>MAGSGKFFVGGNWKCNGTKDSIAKLISDLNSATLEADVDVVVSPPFVYIDQVKSSLTDRIDISGQNSWVGKGGAFTGEISVEQLKDLGCKWVILGHSERRHVIGEKDEFIGKKAAYALSEGLGVIACIGEKLEEREAGKTFDVCFAQLKAFADAVPSWDNIVVAYEPVWAIGTGKVASPQQAQEVHVAVRGWLKKNVSEEVASKTRIIYGGSVNGGNSAELAKEEDIDGFLVGGASLKGPEFATIVNSVTSKKVAA[2x]

Triosephosphate isomerase (TPI) interconverts glyceraldehyde 3-phosphate (G3P) and dihydroxyacetone phosphate (DHAP). One or various cytoplasmic and chloroplast TPIs (cTPI and pdTPI), are present in plant genomes. cTPIs are involved in glycolysis, whereas chloroplast enzymes participate in the Calvin-Benson cycle. The three-dimensional structures of AtTPIs confirm that both enzymes assembled as dimers with asymmetric units containing two monomers that fold into a canonical (β-α)8 or TIM-barrel. In conclusion, our data indicate that the duplicated TPI gene from A. thaliana has suffered two evolutionary fates: the cTPI isoform is susceptible to redox agents, whereas the pdTPI isoform is resistant.

Crystal structures of cTPI and pdTPI were solved at 1.7 and 2.15 Å respectively. The recombinant construct that encodes pdTPI eliminates the first 59 amino acids that correspond to the predicted chloroplast targeting sequence. In pdTPI, residue C15 presents an ASA of 2.8 and 3.3 Å2, whereas residue C89 presents an ASA of 8.2 and 8.5 Å2. In the case of pdTPI, DTNB conjugation indicates that this protein contains 1.6 cysteines per monomer, this number can be associated with local structural fluctuations or breathing motions near buried thiol groups. Previously it has been shown that residue K84 in yeast TPI exhibits breathing motions, since this residue is located at an analogous structural position near pdTPI-C89 it is possible that structural transitions may transiently expose the thiol group of C89 to the solvent. On the other hand, pdTPI was not inhibited by addition of DA but addition of DTT lead to a decrease in the activity of this enzyme. In contrast the addition of GSSG did not induce a significant effect on pdTPI activity in a range of concentrations from 0.87 to 4.3 mM. In the case of pdTPI mutants, a Western blot signal was not detected for the pdTPI-C15S mutant, whereas the intensity of the signal for pdTPI-C89S was similar to that of the wild-type pdTPI. From these loop 3 residues, the only interaction that is different between AtTPIs, is that in cTPI residue M83 makes a hydrophobic interaction with cTPI-C13, whereas in pdTPI residue Q83 makes a H-bond with pdTPI-C15. Our structural data suggest that the H-bond interaction of pdTPI-C15 to pdTPI-Q8 is responsible for decreased reactivity in pdTPI-C15.>[4x]KGPNLTEISKKITESNAVVLAVKEIETLLASIDELATKAIGKKIQQNGGLAVEAGHNGTLLAGAYTISKLITQKLDGLKNSEKLKEKIENAKKCSEDFTKKLEGEHAQLGIENVTDENAKKAILITDAAKDKGAAELEKLFKAVENLAKAAKEMLANSVKELTSP

Outer surface protein C (OspC) plays a pivotal role in mediating tick-to-host transmission and infectivity of the Lyme disease spirochete, Borreliella burgdorferi. OspC is a helical-rich homodimer that interacts with tick salivary proteins, as well as components of the mammalian immune system. OspC consists of four long α-helices, two shorter α-helices (4 and 5), and two short antiparallel β-strands located between α1 and α2 (23, 24). The biologically functional molecule is a dimer (with monomers referred to here as OspC-OspC′) that assumes a knob-shaped structure anchored via an N-terminal lipidated moiety in the spirochete’s outer membrane.

To elucidate the structural basis for B5 IgG’s specificity for OspCA, we solved the crystal structures of recombinant OspCB and OspCK at 1.5-Å and 1.9-Å resolution, respectively, in the P21 space group. OspCB and OspCK each formed homodimers nearly identical to those of OspCA (unbound or bound to B5). Specifically, OspCB and OspCK monomers each consisted of four long α-helices, two shorter α-helices (4 and 5), and a two-stranded β-sheet. The monomeric form of OspCA (with or without B5 Fab bound) was structurally more similar to OspCK than OspCB, with an RMSD of ~0.7 Å for all atoms. By ELISA, B5 IgG reacted with OspCA but had no detectable reactivity with either OspCB or OspCK. Superpositioning the B5-OspCA complex onto OspCB and OspCK revealed additional structural attributes that likely account for B5’s inability to recognize OspCB and OspCK. In OspCB and OspCK, Glu-175 is superposed with OspCA Gly-174. The bulkier and negatively charged Glu-175 side would be expected to clash (sterically and electrostatically) with Trp-100, thereby impeding B5 interaction. In the case of OspCK, divergent primary amino acid sequences at consequential residues further contributed to a lack of B5 recognition. For example, OspCA Lys161 forms a π-cation interaction with B5 Trp-100, which cannot occur in the case of OspCK due to an Ile residue at this position.>[2x]SMEIPSKQIDYRDVFIEFL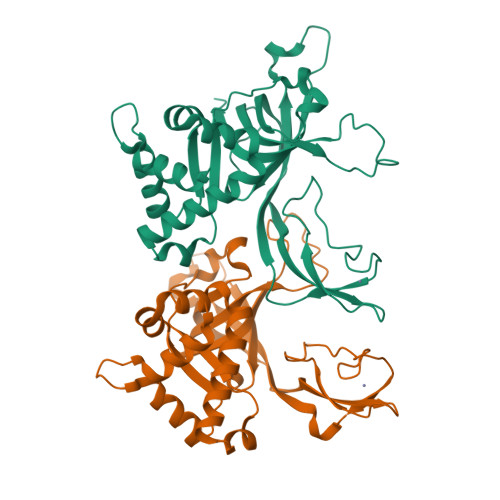TTFKGNNNQNKYIERINELVAYRKKSLIIEFSDVLSFNENLAYEIINNTKIILPILEGALYDHILQLDPTYQRDIEKVHVRIVGIPRVIELRKIRSTDIGKLITIDGILVKVTPVKERIYKATYKHIHPDCMQEFEWPEDEEMPEVLEMPTICPKCGKPGQFRLIPEKTKLIDWQKAVIQERPEEVPSGQLPRQLEIILEDDLVDSARPGDRVKVTGILDIKQDSPVKRGSRAVFDIYMKVSSIEVSQKVL>[2x]MIEAILFDVNGTLAETEELHRRAFNETFAALGVDWFWDR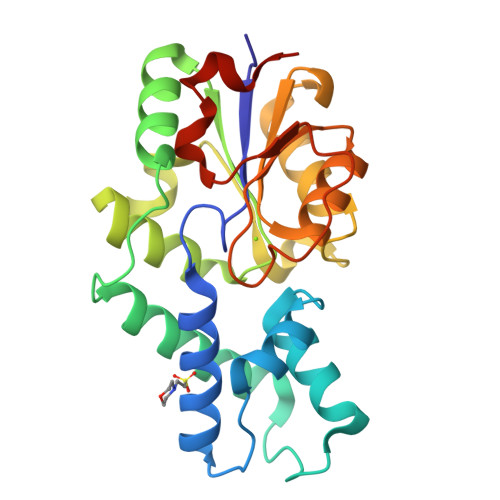EEYRELLTTTGGKERIARFLRHQKGDPAPLPIADIHRAKTERFVALMAEGEIALRPGIADLIAEAKRAGIRLAVATTTSLPNVEALCRACFGHPAREIFDVIAAGDMVAEKKPSPDIYRLALRELDVPPERAVALEDSLNGLRAAKGAGLRCIVSPGFYTRHEEFAGADRLLDSFAELGGLAGLDLTAPVA> HMTIPGRFMTIDKGTFGEYTASTRWPIIIQNAIDDLSKHQETEKSNGTKFEQGEVIKKELKEFRQEIIDRVPLRPFTEE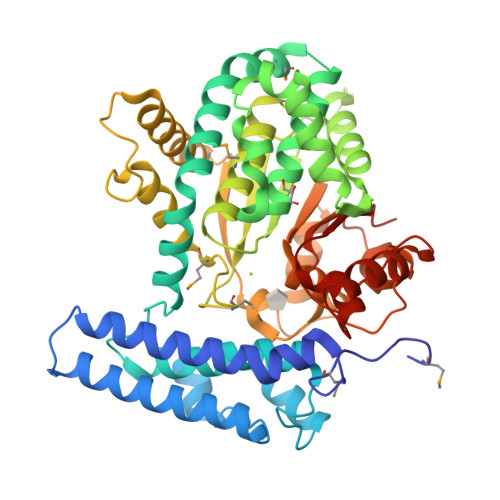EIKIANVPLSFNEYLKKHPEVNWGAVEWLFSEVYLYRRVNVLFQRQCEWAKFDIFNRLKQSTFESSFYGVVELALRYENLLPQLREMKQNPGNEIDDILKVLFKEFIEISLWGNATDLSLLTNATLEDIKSIQGAKARAASESKIVVNDTEKAWEVLTKARADANSREIRVDFVLDNSGFELYADLMLAAFLLQSGLATKCIFHAKDIPYMVSDVMLKDFDILVHDLRDREFFPSGEPSTKESRALDLFAGEMEKFVSSGKIEFREDSFWTTELDYWNLDANETKYHGSILHKDLQKSNLVIFKGDLNYRKLTGDRKWPRTTKWETAIGPLATNGITSLSLRTCKADVQVALPEGLDAKLSQEWEKENPGRGSWWCCSGKWAVICFCSGIHK> M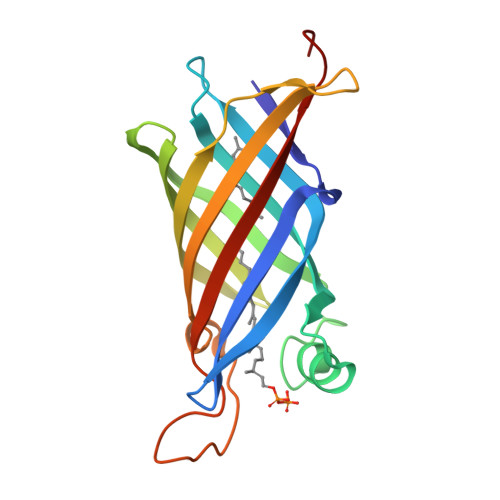KWNLDPSHTSIDFKVRHMGIASVRGSLKVLSGSVETDEAGRPIQVEAVIDAASIATGEPQRDGHLRSADFLHAEQYPEIRFVSTQIEPLGGNRYRIQGNLTIRDITKPVTLEAEVSAPIKDPWGMQRVAASASGQINRKDWNLTWNQVLELGALLVGEEVKFNLEVEAVAPAPVAAQ>AEQKTLHIYNWSDYIAPDTVANFE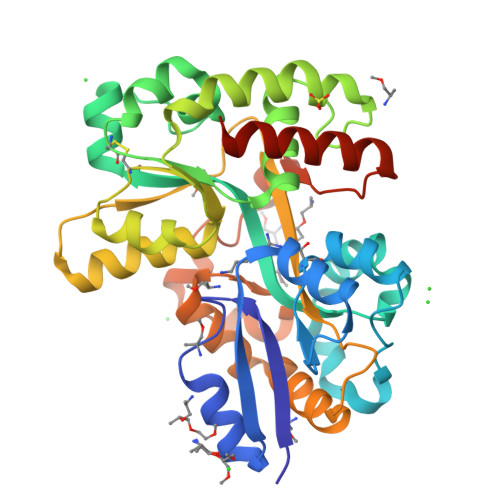KETGIKVVYDVFDSNEVLEGKLMAGSTGFDLVVPSASFLERQLTAGVFQPLDKSKLPEWKNLDPELLKLVAKHDPDNKFAMPYMWATTGIGYNVDKVKAVLGENAPVDSWDLILKPENLEKLKSCGVSFLDAPEEVFATVLNYLGKDPNSTKADDYTGPATDLLLKLRPNIRYFHSSQYINDLANGDICVAIGWAGDVWQASNRAKEAKNGVNVSFSIPKEGAMAFFDVFAMPADAKNKDEAYQFLNYLLRPDVVAHISDHVFYANANKAATPLVSAEVRENPGIYPPADVRAKLFTLKVQDPKIDRVRTRAWTKVKSGKLEHHHHHH[2x]> SNAAPAATPLT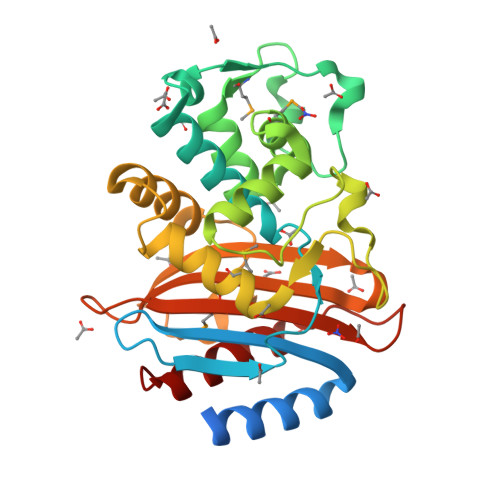ATPTPAAAPATAMQAAPDGARARKELRTLEASFKGRIGAYAVDTATGKTITYRSGERFPLLSTFKAIAAAAVLHKARTSDPGLLNKVVHWTTAELQEHSPVTGKHVKDGMTVARLCEAAITRSDNTAANMLLKQIGGPAGLTAYFHTLKDPVSRLDRWETELNNWSPKEKRDTTTPASMGRDLRAVTTGDALDARDRERLNAWLTANKTGDARIRAGLPKTWTVGDKTGTNSKYGAGNDIAVVWPGKSAAPIIMSIYTNRGAADAAVDDKVIADTAAILARALGKL>[2x]MLPHGLIVSCQALPDEPLHSSFIMSKMALAAYEGGAVGIRANTKEDILAIKETVDLPVIGIVKRDYDHSDVFITATSKEVDELIESQCEVIALDATLQ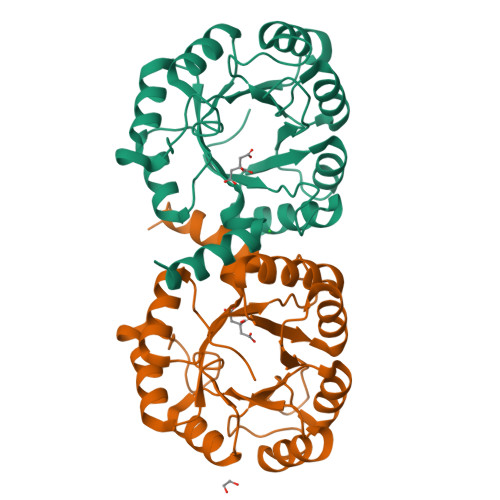QRPKETLDELVSYIRTHAPNVEIMADIATVEEAKNAARLGFDYIGTTLHGYTSYTQGQLLYQNDFQFLKDVLQSVDAKVIAAGNVITPDMYKRVMDLGVHCSVVGGAITRPKEITKRFVQIMED>GNLPPEKKWLGTPIEEMRKMPRCGIHLPSLRPSASHTVTVRVDLLRAGEVPKPFPTHYKDLWDNKHVKMPCSEQNLYPVEDENGERTAGSRWELIQTALLNKFTRPQNLKDAILKYNVAYSKKWDFTALVDFWDKVLEEAEAQHLYQSILPDMVKIALCLPNICTQPIPLLKQKMNHSVTMSQEQIASLLANAFFCTFPRRNAKMKSEYSSYPDINFNRLFEGRSSRKPEKLKTLFCYFRRVTEKKPTGLVTFTRQSLEDFPEWERCEKPLTRLHVTYEGTIEGNGRGMLQVDFANRFVGGGVTGAGLVQEEIRFLINPELIVSRLFTEVLDHNECLIITGTEQYSEYTGYAETYRWARSHEDGSEKDDWQRRCTEIVAIDALHFRRYLDQFVPEKVRRELNKAYCGFLRPGVPSENLSAVATGNWGCGAFGGDARLKALIQILAAAAAERDVVYFTFGDSELMRDIYSMHTFLTERKLDVGKVYKLLLRYYNEECRNCSTPGPDIKLYPFIYHAVESSAET[3x]

Reversal of PARylation is predominantly carried out by poly(ADP-ribose) glycohydrolase (PARG) in nucleus and cytosol, whereas ADP-ribosylhydrolase 3 (ARH3) may play a role in mitochondrial PAR degradation. PARG comprises an N-terminal regulatory/targeting domain and a C-terminal catalytic domain. The mouse PARG catalytic domain has a bean-shaped structure, with the active site in a deep cleft in the middle on the abdominal side.

Among proposed PARG inhibitors, adenosine 5′-diphosphate-(hydroxymethyl)-pyrrolidinediol (ADP-HPD), an analogue of ADPr, is probably the most potent and best studied one, with an IC50 of about 120 nM. Under a new crystallization condition, we obtained a second crystal form (space group P21212) successfully soaked in ADPr and ADP-HPD, and solved the complex structures by molecular replacement. ADPr or ADP-HPD binds to the active site cleft of mPARG. The signature catalytic loop (GGGVTGAGLVQEE) interacts with the ribose ring of ADPr or the pyrrolidine ring of the ADP-HPD. Residue Glu748 forms a hydrogen bond with the 2″-OH, while the key catalytic residue Glu749 side chain carboxyl group is very close to the 1′-OH of the ADPr or the C1″ of the ADP-HPD. The second conserved glycine rich loop (GCGAFGGD) interacts with the diphosphate group of the ADPr or ADP-HPD. Upon binding, the second conserved glycine rich loop (GCGAFGGD) undergoes a major conformational change to tightly interact with the ADP-HPD. The side chain dihedral angle of Phe868 rotates about 90° to form a close contact with the pyrrolidine ring. The side chain dihedral angle of Phe895 rotates about 120° to form parallel π stacking interactions with the adenine ring and subsequently close the deep pocket for the adenine ring. Our PARG structure in complex with ADPr and ADP-HPD suggests that mouse PARG uses a very similar mechanism.> K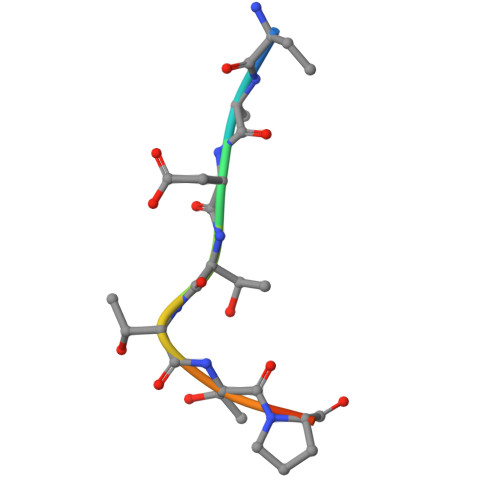ADTTTPTT> MSFRFGQHLIKPSVVFLKTELSFALVNRKPVVPGHVLVCPLRPVERFHDLRPDEVADLFQTTQRVGTVVEKHFHGTSLTFSMQDGPEAGQTVKHVNVHVLPRKAGDFHRNDSIYEELQKHDK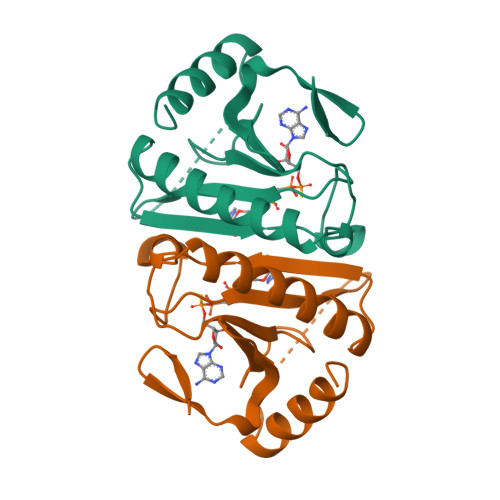EDFPASWRSEEEMAAEAAALRVYFQ>MTVFRQENVDDYYDTGEELGSGQFAVVKKCREKSTGLQYAAKFIKKRRTKSSRRGVSREDIEREVSILKEIQHPNVITLHEVYENKTDVILILELVAGGELFDFLAEKESLTEEEATEFLKQILNGVYYLHSL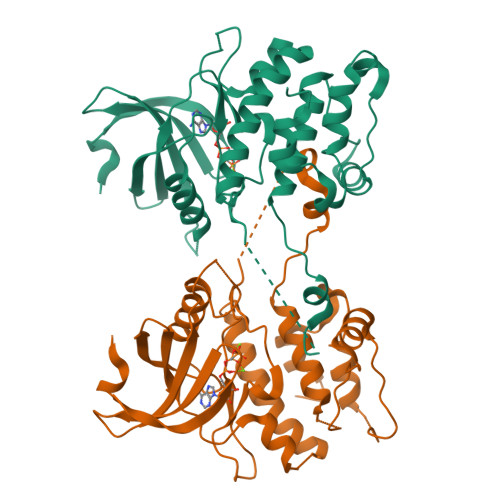QIAHFDLKPENIMLLDRNVPKPRIKIIDFGLAHKIDFGNEFKNIFGTPEFVAPEIVNYEPLGLEADMWSIGVITYILLSGASPFLGDTKQETLANVSAVNYEFEDEYFSNTSALAKDFIRRLLVKDPKKRMTIQDSLQHPWIKPKDTQQALS[4x]>MERPQPDSMPQDLSEALKEATKEVHTQAENAEFMRNFQKGQVTRDGFKLVMASLYHIYVALEEEIERNKESPV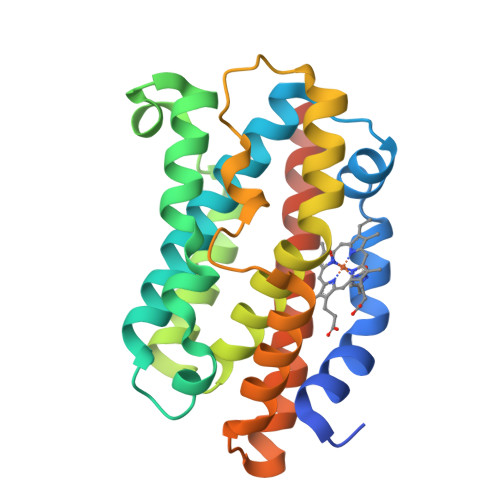FAPVYFPEELHRKAALEQDLAFWYGPRWQEVIPYTPAMQRYVKRLHEVGRTEPELLVAHAYTRYLADLSGGQVLKKIAQKALDLPSSGEGLAFFTFPNIASATKFKQLYESRMNSLEMTPAVRQRVIEEAKTAFLLNIQLFEELQELLTHDTKDQSPSRA[2x]> MDFNLSNSQSDIYESAYRFACDVLDQDAQTRISQKILSTELWKKAAAYGFAHGPVSHQFGGSELGALDTALMIEALGKGSRDIGLSFSLCAHLCACVIPLYRFGSSELKDKYLESLVTGKLIAANAATEPDAGSDIYNMQATAQPCEGGYILNGKKIFITNAPIADVFIIYAKTNPDHGFLGVSAFLIEKGTPGLNVGEVIPKD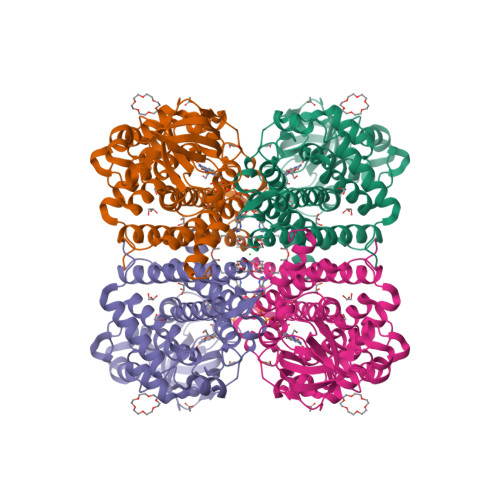CLSNCPWSEIVFNDIFIPQSQRIGMEGAGGAIFHDSMIWEKGCLSALFVGGLARLLETTLEYAKARQQFGKAIGQFQSVSNRIIDMKLRLEQCRLMLYRACWKHDQGQDAEADIAMSKLLISEYAVQSGLDAIQTFGGAAMDQELGLVRHLLNMIPSRIFSGTNDIQKEIIARKLGLRGTSSGSLVPRGSHHHHHHHH>[2x]ASNFDCCLGYTDRILHPKFIVGFTRQLANEG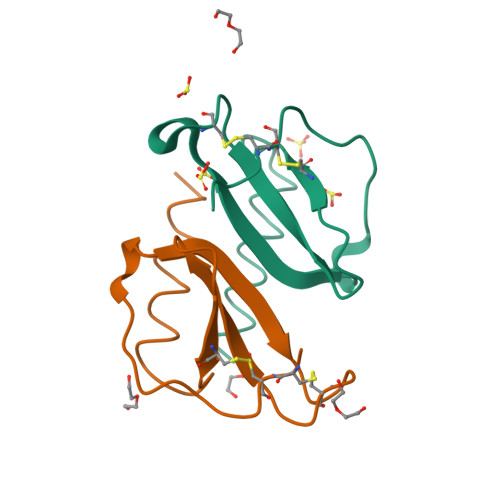CDINAIIFHTKKKLSVCANPKQTWVKYIVRLLSKKVKN>[2x]SN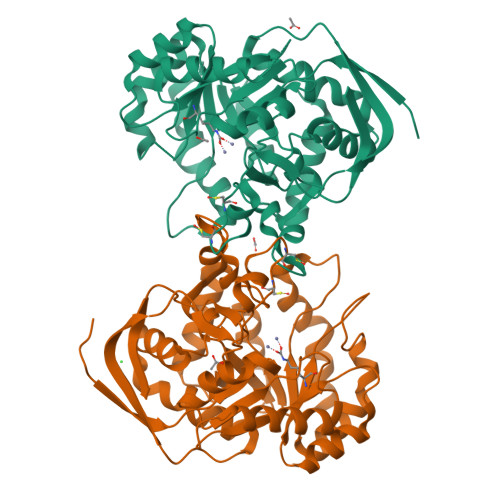AMTTLTITRPDDWHVHLRDGDVLADTVRDISRYNGRALIMPNTVPPVTTTEMALAYRERIMAAQPQAHFEPLMALYLTDNTSPEEIRKAKASGKVVAAKLYPAGATTNSDSGVTSAKNIYPVLQAMQEVGMLLLVHGEVTTHEVDIFDREKTFLDTVLAPIVNDFPQLKIVLEHITTADAVTFVQQAGDNVAATITAHHLLFNRNHMLVGGIRPHFYCLPILKRATHQHALVAAATSGSKKFFLGTDSAPHAKGRKEAACGCAGSYTAHAALELYAEVFEKEGKLENLEAFASFNGPDFYGLPRNQETVTLTKQAWPVAESMPFGSDIVVPIRAGENIEWTVK> MSSTVISRKRRNSTVTEPDSSGETRKQKKSRSDEKSSSSKDGDPQLEFKVLQGYRDLESEMHKGRAQVTRTGDIGVAMDNLNAVDSLFNKVIGIKNNGLFAHDARAMVSISELAQISVRNLKFDDSRSMVNLENIVNSLKRYMLKEHFKLNNIAENRNDLTLAADEQSAADQQEESDGDIDRTPDDNHTDKATSSFKATSMRHSYLQQFSHYNEFSQFNWFRIGALYNTISKNAPITDHLMGPLSIEKKPRVLTQRRRNNDQVGEKITAEKITQHSLNSTQQETTPEQVKKCFKKLSKKLGPEGSINLFKFIIDPNSFSRSIENLFYTSFLIKEGKLLMEHDEE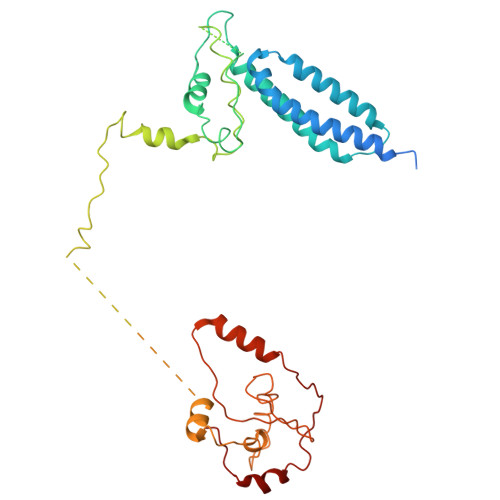GLPTIKIKQSISHTDSRSKEIERQRRRAAHQNHIIFQMDMPTWRKLIKKYNITSPFLD> MTFVDIHAIQTLPYSNINRDDLGSPKTVVYGGKERTRVSSQSWKRAVRHEVEARLGDKAVRTRRIISEIAKRLRERGWDADLADAGARQVVLSVGKKSGIKLEKEKDSEAPATSVLFYLPVPAIDELAAIADEHRDAVAKEAAKKTPKGILPADRITEVLKSRNVSVNLFGRMLAELPSTEVDGAVQFAHAFTVHGTTVEVDFFTAVDDIPKENDHGSGHMNAG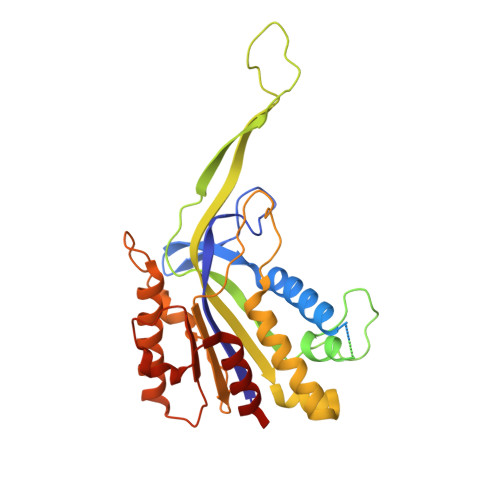QFSAGTFYRYANVNLDRLVENTGDAQTARTAVAEFLRAFLSTVPSGKQNATAAMTLPDLVHIAVRFDRPISFAPAFETALYGSDGYTLRACQELNNYAERLREVWPDDAIRGYATVENKTDLAALGERYDSYPALIDAMVAAAFEGERE> VNNTIVVSIGQAGNQIAASFWKTVCLEHGIDPLTGQTAPGVAPRGNWSSFFSKLGESSSGSYVPRAIMVDLEPSVIDNVKATSGSLFNPANLISRTEGAGGNFAVGYLGAGREVLPEVMSRLDYEIDKCDNVGGIIVLHAIGGGTGSGFGALLIESLKEKYGEIPVLSCAVLPSPQVSSVVTEPYNTVFALNTLRRSADACLIFDNEALFDLAHRKWNIESPTVDDLNLLITEALAGITASMRFSGFLTVEITLRELLTNLVPQPSLHFLMCAFAPLTPPDRSKFEELGIEEMIKSLFDNGSVFAACSPMEGRFLSTAVLYRGIMEDKPLA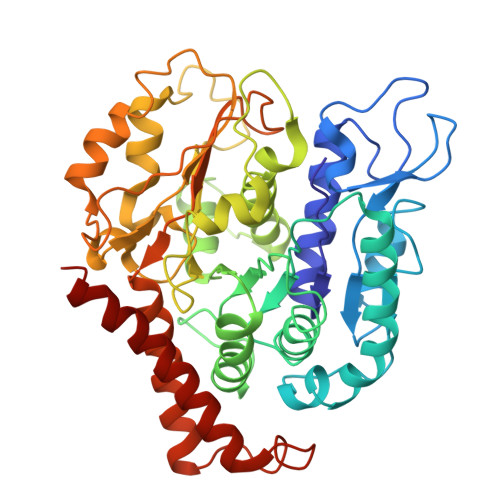DAALAAMREKLPLTYWIPTAFKIGYVEQPGISHRKSMVLLANNTEIARVLDRICHNFDKLWQRKAFANWYLNEGMSEEQINVLRASAQELVQSYQVAEESGA> SGSAKVAFSAIRSTNHEPSEMSNRTMIIYFDQVLVNIGNNFDSERSTFIAPRKGIYSFNF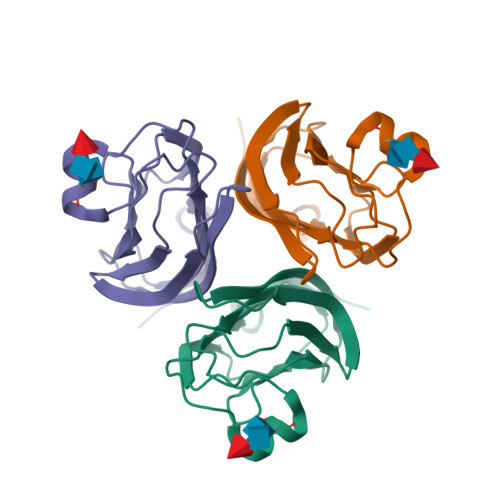HVVKVYNRQTIQVSLMLNGWPVISAFAGDQDVTREAASNGVLIQMEKGDRAYLKLERGNLMGGWKYSTFSGFLVFPLHHHHHH> MGSSHHH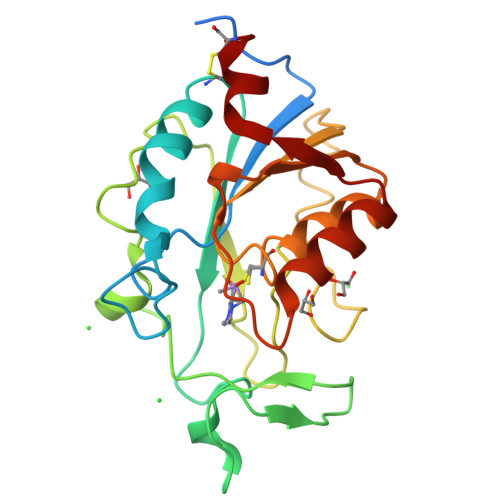HHHSSGENLYFQGHMKMNKQPQNSALVVVDVQNGFTPGGNLAVADADTIIPTINQLAGCFENVVLTQDWHPDNHISFAANHPGKQPFETIELDYGSQVLWPKHCIQGTHDAEFHPDLNIPTAQLIIRKGFHAHIDSYSAFMEADHTTMTGLTGYLKERGIDTVYVVGIATDFCVAWTALDAVKQGFKTLVIEDACKGIDLNGSLEQAWQTMQQQGVVRIQSTDLLNEC3-(5-AMINO-7-HYDROXY-[1,2,3]TRIAZOLO[4,5-D]PYRIMIDIN-2-YL)-N-[2-(2-(HYDROXYMETHYL-PHENYLSULFANYL)-BENZYL]-BENZAMIDE 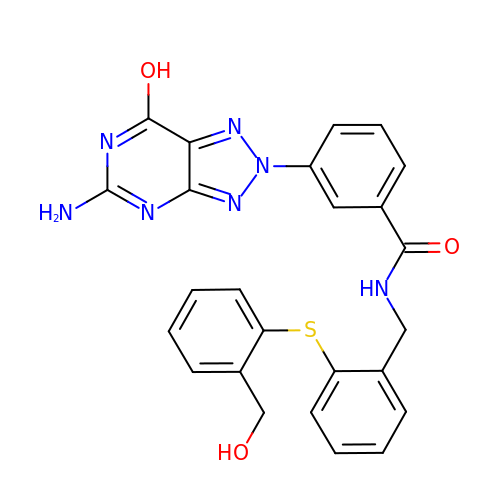| C25 H21 N7 O3 S | IXDQOBDHBWEZOH-UHFFFAOYSA-N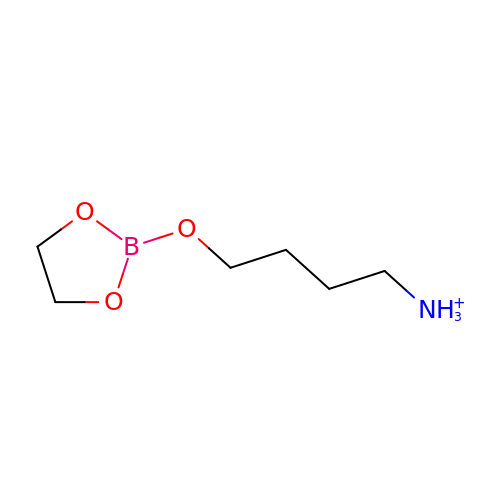4-(1,3,2-DIOXABOROLAN-2-YLOXY)BUTAN-1-AMINIUM | C6 H15 B N O3 | KTZDASPSWBAPAR-UHFFFAOYSA-O> MQLKGKTAIVTGSSRGLGKAIAWKLGNMGANIVLNGSPASTSLDATAEEFKAAGINVVVAKGDVKNPEDVENMVKTAMDAFGRIDILVNNAGITRDTLMLKMSEKDWDDVLNTNLK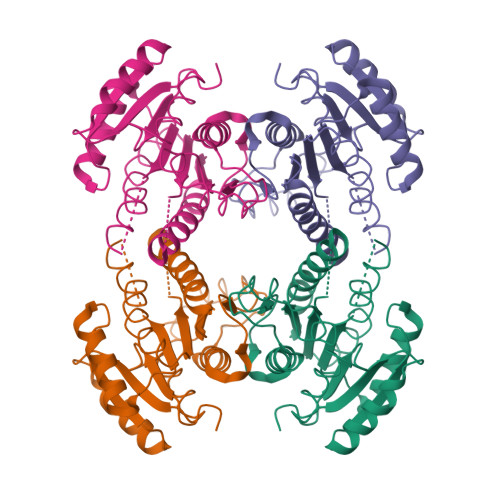SAYLCTKAVSKIMLKQKSGKIINITSIAGIIGNAGQANYAASKAGLIGFTKSIAKEFAAKGIYCNAVAPGIIKTDMTDVLPDKVKEMYLNNIPLKRFGTPEEVANVVGFLASDDSNYITGQVINIDGGLVM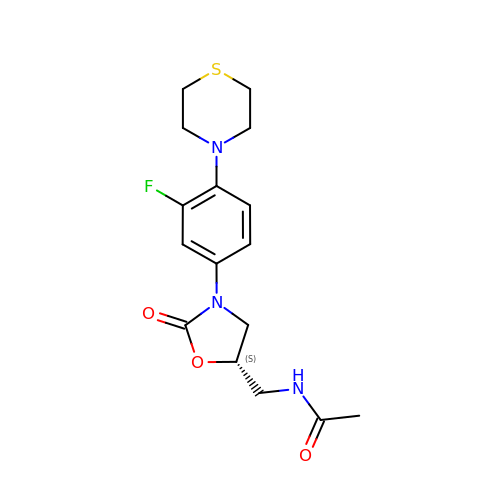~{N}-[[(5~{S})-3-(3-fluoranyl-4-thiomorpholin-4-yl-phenyl)-2-oxidanylidene-1,3-oxazolidin-5-yl]methyl]ethanamide | C16 H20 F N3 O3 S | FNDDDNOJWPQCBZ-ZDUSSCGKSA-N>[2x]MTADELVFFVNGKKVVEKNADPETTLLVYLRRKLGLCGTKLGCGEGGCGACTVMISKYDRLQNKIVHFSVNACLAPICSLHHVAVTTVEGIGNTQKLHPVQERIARSHGSQCGFCTPGIVMSMYTLLRNQPEPTVEEIENAFQGNLCRCTGYRPILQGFRTFAKDGGCCGGSGNNPNCCMNQTKDQTVSLSPSLFNPEDFKPLDPTQEPIFPPELLRLKDTPQKKLRFEGERVTWIQASTMEELLDLKAQHPDAKLVVGNTEIGIEMKFKNMLFPLIVCPAWIPELNSVVHGPEGISFGASCPLSLVESVLAEEIAKLPEQKTEVFRGVMEQLRWFAGKQVKSVASIGGNIITASPISDLNPVFMASGAKLTLVSRGTRRTVRMDHTFFPGYRKTLLRPEEILLSIEIPYSKEGEFFSAFKQASRRENDIAKVTSGMRVLFKPGTIEVQELSLCFGGMADRTISALKTTPKQLSKSWNEELLQSVCAGLAEELQLAPDAPGGMVEFRRTLTLSFFFKFYLTVLQKLGRADLEDMCGKLDPTFASATLLFQKDPPANVQLFQEVPKDQSEEDMVGRPLPHLAANMQASGEAVYCDDIPRYENELSLRLVTSTRAHAKITSIDTSEAKKVPGFVCFLTAEDVPNSNATGLFNDETVFAKDEVTCVGHIIGAVVADTPEHAQRAARGVKITYEDLPAIITIQDAINNNSFYGSEIKIEKGDLKKGFSEADNVVSGELYIGGQEHFYLETNCTIAVPKGEAGEMELFVSTQNTMKTQSFVAKMLGVPDNRIVVRVKRMGGGFGGKETRST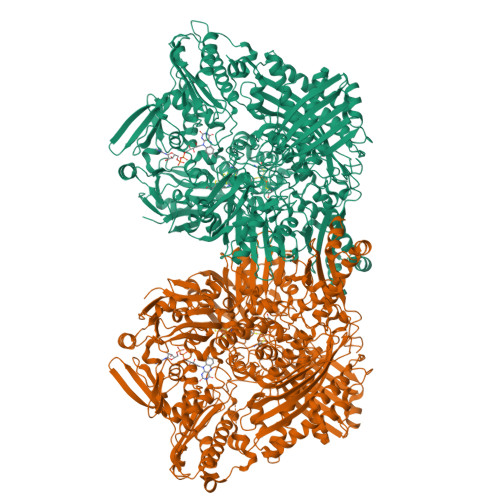VVSTALALAAHKTGRPVRCMLDRDEDMLITGGRHPFLAKYKVGFMKTGTVVALEVAHFSNGGNTEDLSRSIMERALFHMDNAYKIPNIRGTGRICKTNLPSNTAFRGFGGPQGMLIAEYWMSEVAITCGLPAEEVRRKNMYKEGDLTHFNQKLEGFTLPRCWDECIASSQYLARKREVEKFNRENCWKKRGLCIIPTKFGISFTLPFLNQGGALVHVYTDGSVLLTHGGTEMGQGLHTKMVQVASRALKIPTSKIHISETSTNTVPNTSPTAASASADLNGQGVYEACQTILKRLEPFKKKKPTGPWEAWVMDAYTSAVSLSATGFYKTPNLGYSFETNSGNPFHYFSYGVACSEVEIDCLTGDHKNLRTDIVMDVGSSLNPAIDIGQVEGAFVQGLGLFTMEELHYSPEGSLHTRGPSTYKIPAFGSIPIEFRVSLLRDCPNKRAIYASKAVGEPPLFLASSIFFAIKDAIRAARAQHGDNAKQLFQLDSPATPEKIRNACVDQFTTLCVTGVPENCKSWSVRI> APKRERKTIRIRDPNQGGKDIT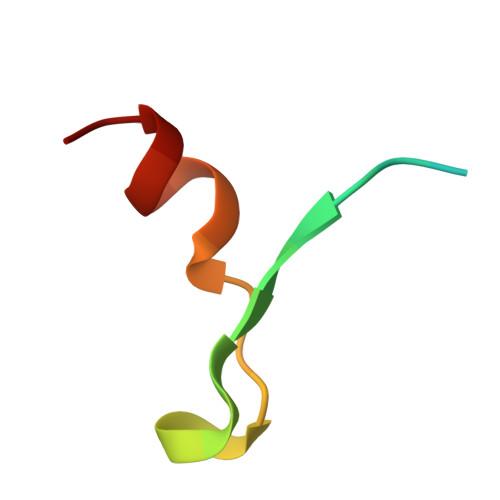EEIMSG> HHHHHHGSATIDGIIQGSVHSALTGESYGESVKQAVILNVVGGGDSIADPLSPGENDMVHRLKRLEDEQKGEIIRTKHNAQVIAKFGRDLEDVYKFASREHKVGEEEEDQIQMLEKALRAYGNVVKVEGESVQKLAKALRAEEEERTDEETRMIGEYRDKIDALSKAIEIEREGLQDEAIQEIAGMSAEVLEAAAEEVPIFGAGVATSIATARAIEGAYKLKAVITALTGIDLSHMTTPKIQPKTLEAILDAPGGNVTDLMLTRGLDSKIDKINENLAEVEHMQTSILPRIKKAIEEDRDEITNWSPKRIHPKSVQRFRVPRMQTPSIHIYAAPWDSDSVFIFHVISPHHLNESFFLGFDLEIEYVHYEDLAQHWHSLGAAQEVTGRTFREAYREFFNLASRSTMASDIHKKRLQRSRMSHPIYLGVHNYELSYIAIKSNAMQLVTDEDLQKHVLRGPLHFQRRVIMAALKYGVKVMSRADDIAMMLRDA

Bluetongue virus (BTV) is transmitted by blood-feeding midges (Culicoides sp.), causes haemorrhagic diseases in livestock and is responsible for considerable global economic losses.It is an unenveloped icosahedral virus, belonging to the Orbivirus genus of the family Sedoreoviridae, with a multilayer capsid enclosing a segmented double-stranded RNA (dsRNA) genome. The inner two capsid layers (composed of VP3 and VP7) comprise a core particle which remains intact following infection, whilst the outer layer contains two proteins, VP2 and VP5. VP2 is the attachment protein and protrudes from the virion surface, whilst VP5 is implicated in membrane penetration. Protein VP5 forms part of the outer layer of BTV, with two symmetric trimers of VP5 fitting like pegs into pits on the underlying core.

Here we characterise VP5 at two pHs by crystallography to provide a detailed analysis of the pH dependent structural changes and consider the consequences at the virion level. The low pH form was solved in the native state and refined at 2.2 Å. The low pH conformation at 2.2 Å provides a precise description of this state, presumed to be primed for host membrane engagement. Since the two N-terminal helices are deleted from the construct the crystal structure begins at the H4 helix (secondary structure numbering follows that defined for the high pH conformation), which lies against the body of the subunit, following which the chain turns to run upwards away from the body of the subunit in an extended helix, H5 (residues 90 to 137). Interestingly the electron density for this extended helix is clear, allowing a reliable model to be built, whereas the density in the cryo-EM reconstruction (EMDB 24684) fades quickly away from the main body of the VP5 subunit, despite which the cryo-EM model is similar to the X-ray structure in this region. Likewise the low pH structure confirms the extended helical protrusion that was inferred but poorly resolved in the previous cryo-EM structure. There are some differences between the structures in the virion and in the crystal, for instance in the low pH crystal form the so called dagger domain (residues 410–421) cannot follow the path seen in the virus, due to clashes with symmetry molecule in the crystal. Low pH triggers a major conformational change in VP5 which enables the penetration of the membrane via the extended helical structure. In summary we show that VP5 in isolation undergoes essentially the same changes with pH as seen in the virus and confirm the helical transition to produce spikes radiating from the virus surface. This indicates that VP5 is a pH driven motor during cell entry.> MDLSELERDNTGRCRLSSPVPAVCRKEPCVLGVAEAGRGPVLGPMVYAICYCPLPRLADLEALKVADSKTLLESERERLFAKMEDTDFVGWALDVLSPNLISTSMLGRVKYNLNSLSHDTATGLIQYALDQGVNVTQVFVDTVGMPETYQARLQQSFPGIEVTVKAKAAALYPVVSAASICAKVARDQAVKKWQFVEKLQDLDTDYGSGYPNDPKTKAWLKEHVEPVFGFPQFVRFSWRTAQTILEKEAEDVIWEDSASENQEG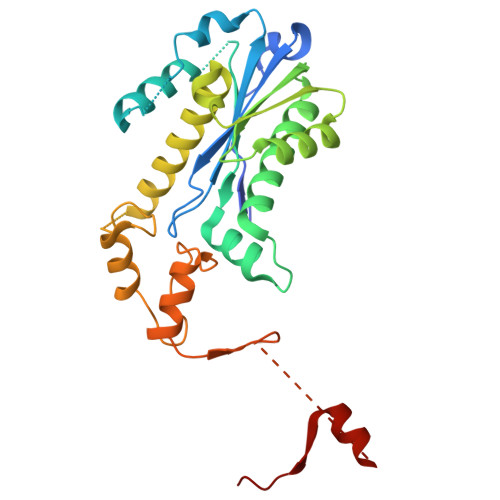LRKITSYFLNEGSQARPRSSHRYFLERGLESATSL>VVTLGYWDIRGLAHAIRLLLEYTETPYQERRYKAGPAPDFDPSDWTNEKEKLGLDFPNLPYLIDGDVKLTQSNAILRYIARKHNMCGETEVEKQRVDVLENHLMDLRMAFARLCYSPDFEKLKPAYLELLPGKLRQLSRFLGSRSWFVGDKLTFVDF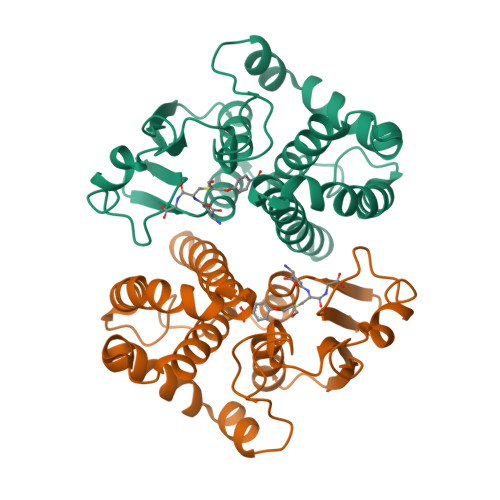LAYDVLDQQRMFVPDCPELQGNLSQFLQRFEALEKISAYMRSGRFMKAPIFWYTALWNNKKE[4x]>[4x]MGKRLKMATIGGGSSYTPELVEGLIKRYHELPVGELWLVDIPEGKEKLEIVGALAKRMVEKAGVPIEIHLTLDRRRALEGADFVTTQFRVGGLEARAKDERIPLKYGVIGQETNGPGGLFKGLRTIPVILDIIRDMEELCPDAWLINFTNPAGMVTEAVLRYTKQEKVVGLCNVPIGMRMGVAKLLGVDADRVHIDFAGLNHMVFGLHVYLDGVEVTEKVIDLVAHPDRSGVTMKNIVDLGWEPDFLKG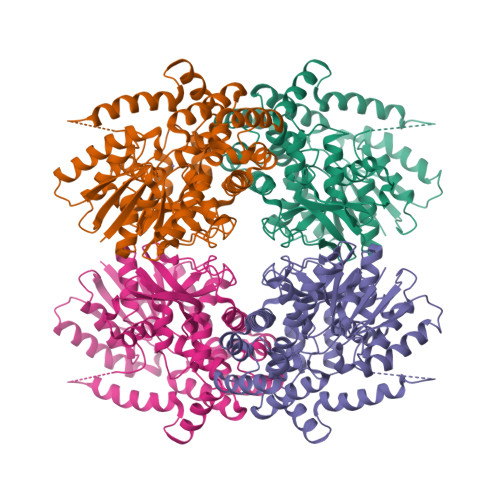LKVLPCPYHRYYYQTDKMLAEELEAAKTKGTRAEVVQQLEKELFELYKDPNLAIKPPQLEQRGGAYYSDAACSLISSIYNDKRDIQPVNTRNNGAIASIPPESAVEVNCVITKDGPKPIAVGDLPVAVRGLVQQIKSFERVAAEAAVTGDYQTALVAMTINPLVPSDTIAKQMLDEMLEAHKEHLPQFFKQAKTVAGN>[2x]MGDIMLIILTGLPGVGKSTFSKNLAKILSKNNIDVIVLGSDLIRESFPVWKEKYEEFIKKSTYRLIDSALKNYWVIVDDTNYYNSMRRDLINIAKKYNKNYAIIYLKASLDVLIRRNIERGEKIPNEVIKKMYEKFDEPGKKYKWDEPFLIIDTTKDIDFNEIAKKLIEKS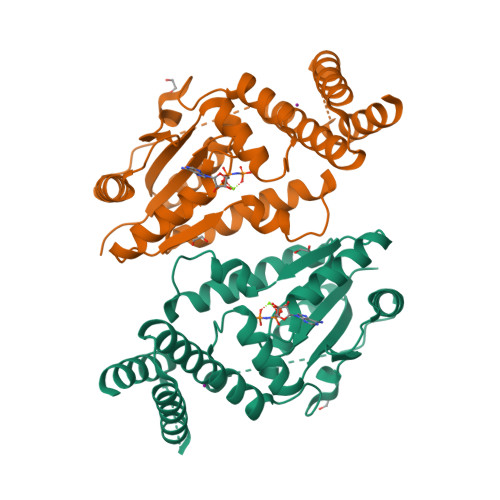KEIPKFYVLEENKNKNNNISDKIDKETRKIVSEYIKSKKLDKDKIKEVVELRKEFLKKIKKMEEVDADRVLKEFKDLLNSYLEHHHHHH>[6x]MMFGRFTERAQKVLALAQEEALRLGHNNIGTEHILLGLVREGEGIAAKALQALGLGSEKIQKEVESLIGRGQEMSQTIHYTPRAKKVIELSMDEARKLGHSYVGTEHILLGLIREGEGVAARVLNNLGVSLNKARQQVLQLLGSNETGSSAAGTNSNANTPTLDSLARDLTAIAKEDSLDPVIGRSKEIQRVIEVLSRRTKNNPVLIGEPGVGKTAIAEGLAQQIINNEVPEILRDKRVMTLDMGTKYRGEFEDRLKKVMDEIRQAGNIILFIDAAIDASNILKPSLARGELQCIGATTLDEYRKYIEKDAALERRFQPIQVDQPSVD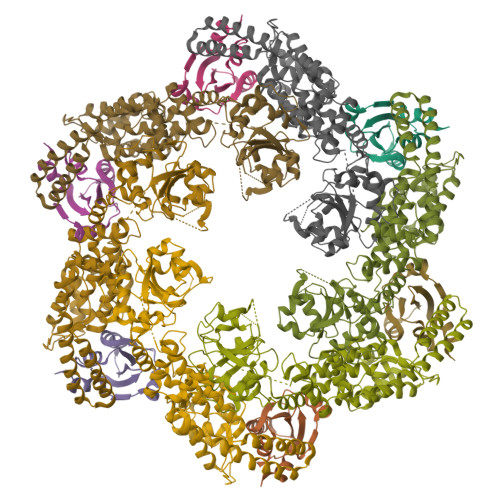ESIQILQGLRDRYEAHHRVSITDDAIEAAVKLSDRYISDRFLPDKAIDLIDEAGSKVRLRSFTTPPNLKELEQKLDEVRKEKDAAVQSQEFEKAASLRDTEQRLREQVEDTKKSWKEKQGQENSEVTVDDIAMVVSSWTG;>[6x]EEKEQKLQFVLRFGDFEDVISLSKLNVNGSKTTLYSFENRYYLYVDFCNMTDEEVENQLSILLEYATESSISIHRLEEYGKLIISEHALETIKKHFAS>[2x]VSASPLKVAVTGAAGQIGYSLLFRLASGSLLGPDRPIELRLLEIEPALQALEGVVMELDDCAFPLLSGVEIGSDPQKIFDGVSLALLVGARPRGAGMERSDLLEANGAIFTAQGKALNAVAADDVRVGVTGNPANTNALIAMTNAPDIPRERFSALTRLDHNRAISQL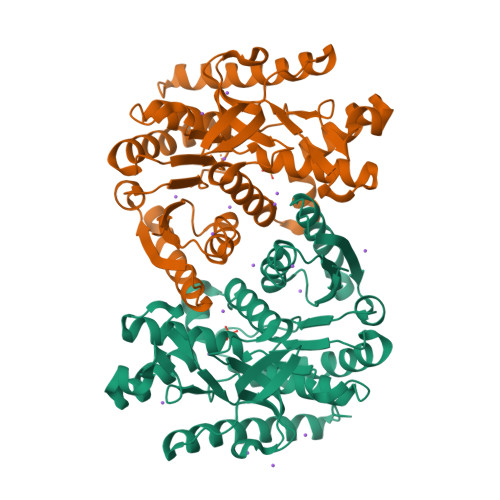AAKTGAAVTDIKKMTIWGNHSATQYPDLFHAEVAGKNAAEVVNDQAWIEDEFIPTVAKRGAAIIDARGASSAASAASATIDAARDWLLGTPADDWVSMAVVSDGSYGVPEGLISSFPVTTKGGNWTIVSGLEIDEFSRGRIDKSTAELADERSAVTELGLIA> MDPLTVYKNSVKQQIDSADLLVANLVNENFVLSEKLDTKATEIKQLQKQIDSLNAQVKEL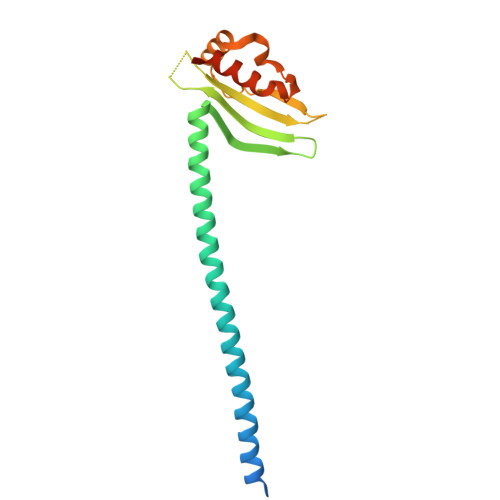KTQTSQQAENSEVIKDLYEYLCNVRVHKSYEDDSGLWFDISQGTHSGGSSDDYSIMDYKLGFVKGQAQVTEVIYAPVLKQRSTEELYSLQSKLPEYLFETLSFPLSSLNQFYNKIAKSLNKKREKKDETE>SNAMNRLKNMSKYSDAKELAS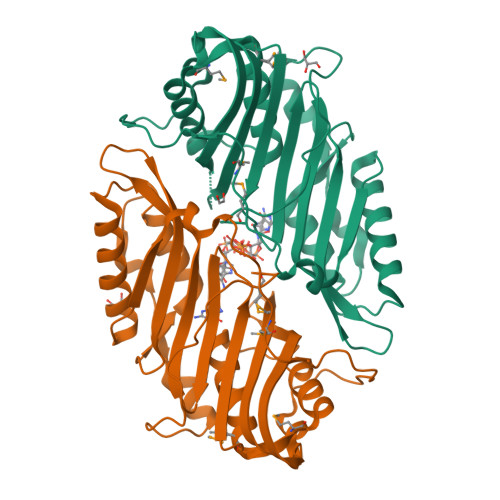LTLGKKTEYANQYDPSLLQPVPRSLNRNDLHLSATLPFQGCDIWTLYELSWLNQKGLPQVAIGEVSIPATSANLIESKSFKLYLNSYNQTRFASWDEVQTRLVHDLSACAGETVTVNVKSLNEYTAEPIVTMQGECIDDQDIEIANYEFDDALLQGAAQGEEVSEVLHSHLLKSNALITNQPDWGSVEIAYHGAKMNREALLRYLVSFREHNEFHEQCVERIFTDIMRYCQPQSLTVYARYTRRGGLDINPFRSSHQSAPNHNQRMARQ[4x]>[8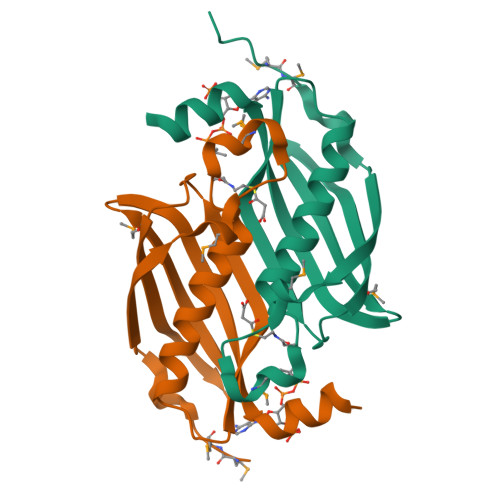x]MGSDKIHHHHHHMMDFDFLEGKRLTEDVALDETMVWNEDIEMLDLHLVATSALIGVVHRVSYELLSRYLPNDYTAVVVETLARHVKAVPTGTRVAVGVRVVGVVGNRVKFRGIVMSGDEKILEAEFVRAIVPREKLRRLALEKAEKTSRLFGI>MSSGLYLYGIFPDPIPETVTLQGLDSQLVYSQIIDGFTFLYSEAKQEKYLASRRNLISHEKVLEQAMHAGFRTLLPLRFGLVVKNWETVVTQLLQPYKAQLRELFQKLAGRREVSVKIFWDSKAELQAMMDSHQDLKQKRDQMEGKALSMEEVIHIGQLIESNLLSRKESIIQVFFDELKPLADEVIESDPMTEDMIYNAAFLIPWENESIFSQQVESIDHKFDERLRIRYNNFTA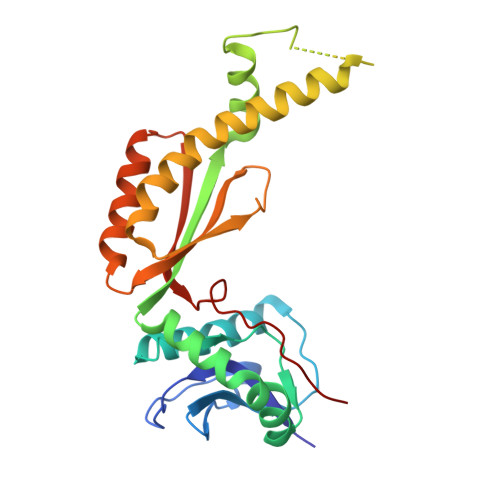PYTFAQISHHHHHH[2x]 N7-(3,4-difluorobenzyl) guanosine 5'-monophosphate | C17 H19 F2 N5 O8 P | 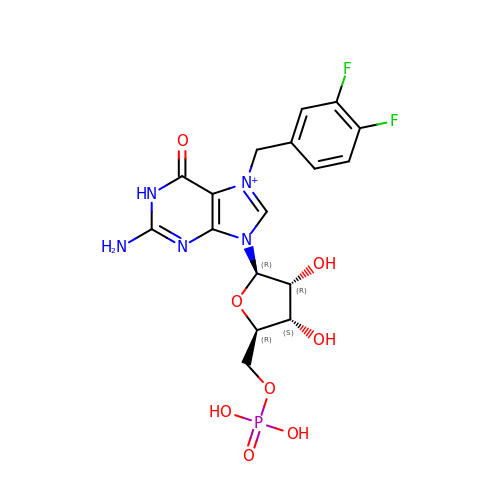BIHPVAUGYOUOAQ-XNIJJKJLSA-O>GAMDSPSPPPALLEKVFQYIDLHQDEFVQTLKEWVAIESDSVQPVPRFRQELFRMMAVAADTLQRLGARVASVDMGPQQLPDGQSLPIPPVILAELGSDPTKGTVCFYGHLDVQPADRGDGWLTDPYVLTEVDGKLYGRGATDNKGPVLAWINAVSAFRALEQDLPVNIKFIIEGMEEAGSVALEELVEKEKDRFFSGVDYIVISDNLWISQRKPAITYGTRGNSYFMVEVKCRDQDFHSGTFGGILHEPMADLVALLGSLVDSSGHILVPGIYDEVVPLTEEEINTYKAIHLDLEEYRNSSRVEKFLFDTKEEILMHLWRYPSLSIHG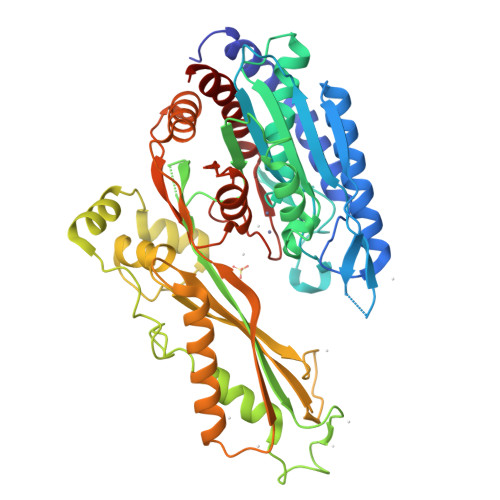IEGAFDEPGTKTVIPGRVIGKFSIRLVPHMNVSAVEKQVTRHLEDVFSKRNSSNKMVVSMTLGLHPWIANIDDTQYLAAKRAIRTVFGTEPDMIRDGSTIPIAKMFQEIVHKSVVLIPLGAVDDGEHSQNEKINRWNYIEGTKLFAAFFLEMAQLH[2x]>MEEPEEPADSGQSLVPVYIYSPEYVSMCDSLAKIPKRADMVHSLIEAYALHKQMRIVKPKVASMEEMATFHTDAYLQHLQKVSQEGDDDHPDSIEYGLGYDCPATEGIFDYAAAIGGATITAAQCLIDGMCKVAINWSGGWHHAKKDEASGFCYLNDAVLGILRLRRKFERILYVDLDLHHGDGVEDAFSFTSKVMTVSLHKFSPGFFPGTGDVSDVGLGKGRYYSVNVPIQDGIQDEKYYQICESVLKEVYQAFNPKAVVLQLGADTIAGDPMCSFNMTPVG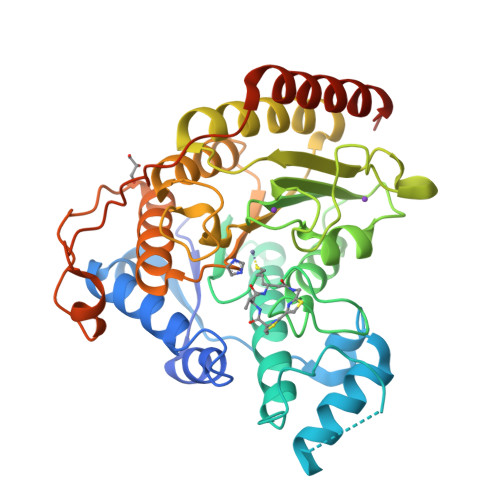IGKCLKYILQWQLATLILGGGGYNLANTARCWTYLTGVILGKTLSSEIPDHEFFTAYGPDYVLEITPSCRPDRNEPHRIQQILNYIKGNLKHVVIEGRGSHHHHHH[2x]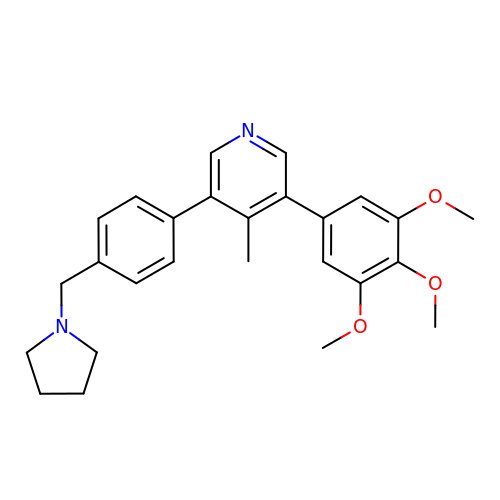4-methyl-3-[4-(pyrrolidin-1-ylmethyl)phenyl]-5-(3,4,5-trimethoxyphenyl)pyridine | C26 H30 N2 O3 | LRZCFVDFECJERV-UHFFFAOYSA-N> MELAAGSFSEEQFWEACAELQQPALAGADWQLLVETSGISIYRLLDKKTGLYEYKVFGVLEDCSPTLLADIYMDSDYRKQWDQYVKELYEQECNGETVVYWEVKYPFPMSNRDYVYLRQRRDLDMEGRKIHVILARSTSMPQLGERSGVIRVKQYKQSLAIESDGKKGSKVFMYYF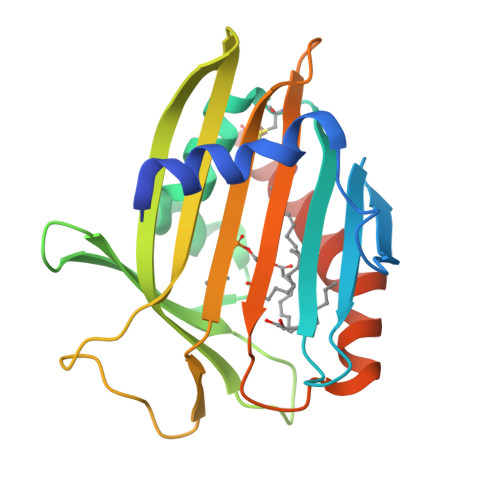DNPGGQIPSWLINWAAKNGVPNFLKDMARACQNYLKKT>MKKILIIGGVAGGASAAARARRLSETAEIIMFERGEYVSFANCGLPYHISGEIAQRSALVLQTPESFKARFNVEVRVKHEVVAIDRAAKLVTVRRLLDGSEYQESYDTLLLSPGAAPIVPPIPGVDNPLTHSLRNIPDMDRILQTIQMNNVEHATVVGGGFIGLEMMESLHHLGIKTTLLELADQVMTPVDREMAGFAHQAIRDQGVDLRLGTALSEVSYQVQTHVASDAAGEDTAHQHIKGHLSLTLSNGELLETDLLIMAIGVRPETQLARDAGLAIGELGGIKVNAMMQTSDPAIYAVGDAVEEQDFVTGQACL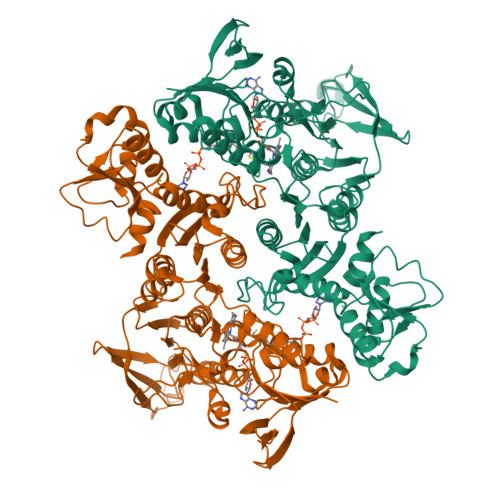VPLAGPANRQGRMAADNMFGREERYQGTQGTAICKVFDLAVGATGKNEKQLKQAGIAFEKVYVHTASHASYYPGAEVVSFKLLFDPVKGTIFGAQAVGKDGIDKRIDVMAVAQRAGMTVEQLQHLELSYAPPYGSAKDVINQAAFVASNIIKGDATPIHFDQIDNLSEDQLLLDVRNPGELQNGGLEGAVNIPVDELRDRMHELPKDKEIIIFSQVGLRGNVAYRQLVNNGYRARNLIGGYRTYKFAS[2x]> SETDDLKWTERLPECPVYRPTKEEFEDPLTYLQKIFPEASKYGICKIVSPLTATVPAGAVLMKEKSNFKFTTRVQPLRLAEWDSDDKVTFFMSGRTYTFRDYEKMANKVFARRYCSGGSLPDSFLEKEFWKEIACGKTETVEYACDVDGSAFSSAPGDPLGSSKWNLNKVSRLPKSTLRLLETSIPGVTEPMLYIGMLFSMFAWHVEDHYLYSINYQHCGASKTWYGIPGSAALKFEKVVKECVYNDDILSTNGEDGAFDVLLGKTTIFPPKTLLDHNVPVYKAVQKPGEFVVTFPRAYHAGFSHGFNCGEAVNFAMGDWFPFGAIASCRYAHLNRVPLLPHEELICKEAMLLNSSSKSENLDLTPTELSGQR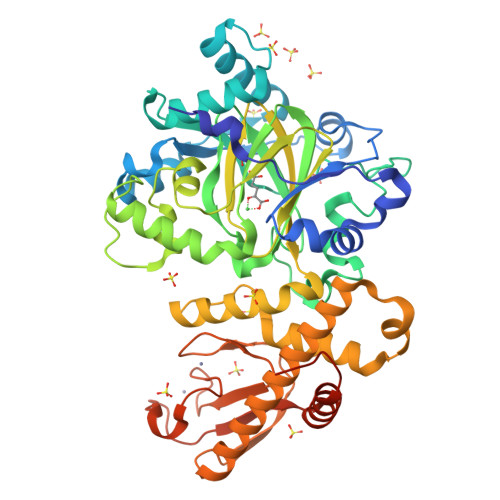SIKTAFVHLIRFLHLARWSLMKSGLCTGLVSNTYGTIVCSLCKRDCYLAFINCECYSHPVCLRHDVKKLDLPCGTTHTLYLRDNIEDMEAAAMKFEKEDGVSDLITTDEDLYKYPSS>MDLKIKNKVCIITGGAKGIGYGIAKLWASEGGIPVIFSRSMPKEHDKELKKLSSEYEFYEIDLKNYEQIEKLVKKVAIKHGGIYALVNNAGTNDNLHIENTSTQDLIKSYENNLFHYYTMTKECLPYIKKEQGSILNIVSKTGITGQGRTSAYASAKAAQMGFTREWACAFAKDNVRVNAIAPAEVMTPLYEKWLQNFPNPKEQ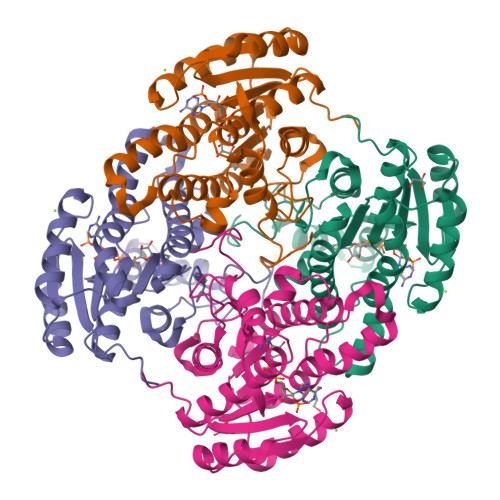YEKIAKAIPLGHRFTTIEEIANTAVFTLSPLASHTTGQILMPDGGYVHLDRALNWDENTRGHHHHHH[4x]> ALSISQVAFEHHRTALGIGETQPRVSWRFDGNVSDWEQRAYEIEVKRAGHDADVFRSESSDSVLVPWPSSPLQSGEEATVRVRSFGSDGQHDTPWSDAVTVEPGLLTPDDWHDAVVIASDRPTEVDATHRPIQFRKEFSVDDSYVSARLYITALGLYEARINDQRVGDHVMAPGWQSYQYRHEYNTYDVTDLLKQGPNAIGVTVGEGWYSGRIGYDGGKRNIYGDTLGLLSLLVVTKSDGSKLYIPSDSSWKSSTGPIISSEIYDGEEYDSRLEQKGWSQVGFNSTGWLGTHELSFPKERLASPDGPPVRRVAEHKLANVFSSASGKTVLDFGQNLVGWLRIRVKGPKGQTIRFVHTEVMENGEVATRPLRQAKATDHFTLSGEGVQEWEPSFTYHGFRYVQVDGWPADTPLDENSVTAIVVHSDMERTGYFECSNPLISKLHENILWSMRGNFFSIPTDCPQRDERLGWTGDIHAFSRTANFIYDTAGFLRAWLKDARSEQLNHSYSLPYVIPNIHGNGETPTSIWGDAIVGVPWQLYESFGDKVMLEEQYGGAKDWVDKGIVRNDVGLWDRSTFQWADWLDPKAPADDPGDATTNKYLVSDAYLLHSTDMLANISTSLSKGEEASNYTEWHAKLTKEFQKAWITSNGTMANETQTGLALPLYFDLFPSAEQAQSAAKRLVNIIKQNDYKVGTGFAGTHLLGHTLSKYGESDAFYSMLRQTEVPSWLYQVVMNGTTTWERWDSMLPNGSINPGQMTSFNHYAVGSVGSWLHEVIGGLSPAEPGWRRINIEVVPGGDLQQASTKFLTPYGMASTKWWLDGQDQSCGGFDFHLVAEVPPNTRATVVLPGKGG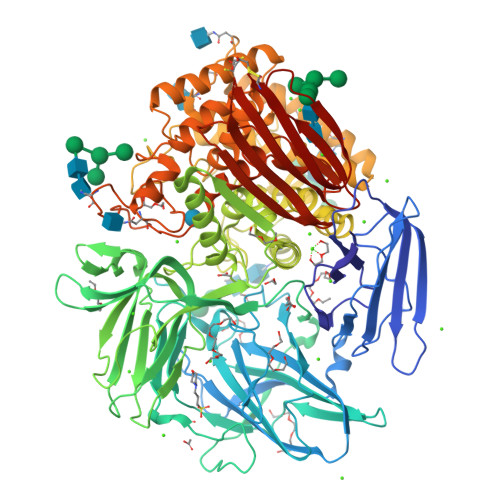EKVDVGSGVHEYHVRCVKL> MIFSDWPWRHWRQVRGETIALRLNDEQLNWRELCARVDELASGFAVQGVVEGSGVMLRAWNTPQTLLAWLALLQCGARVLPVNPQLPQPLLEELLPNLTLQFALVPDGENTFPALTSLHIQLVEGAHAATWQPTRLCSMTLTSGSTGLPKAAVHTYQAHLASAQGVLSLIPFGDHDDWLLSLPLFHVSGQGI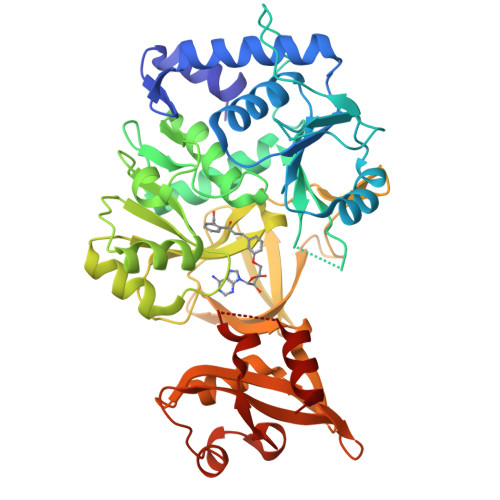MWRWLYAGARMTVRDKQPLEQMLAGCTHASLVPTQLWRLLVNRSSVSLKAVLLGGAAIPVELTEQAREQGIRCFCGYGLTEFASTVCAKEADGLADVGSPLPGREVKIVNNEVWLRAASMAEGYWRNGQLVSLVNDEGWYATRDRGEMHNGKLTIVGRLDNLFFSGGEGIQPEEVERVIAAHPAVLQVFIVPVADKEFGHRPVAVMEYDHESVDLSEWVKDKLARFQQPVRWLTLPPELKNGGIKISRQALKEWVQRQQ> TKFSDNYDVKEELGKGAFSVVRRCVHKTTGLEFAAKIINTKKLSARDFQKLEREARICRKLQHPNIVRLHDSIQEESFHYLVFDLVT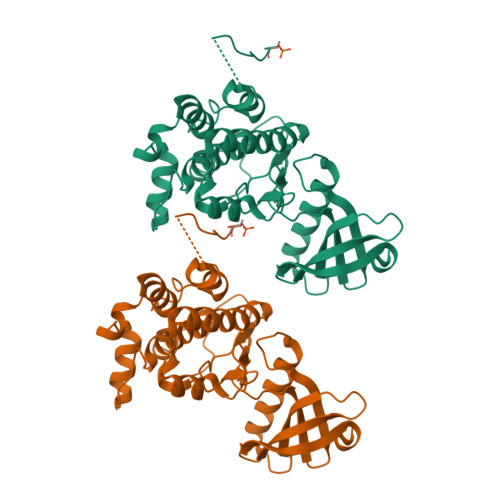GGELFEDIVAREFYSEADASHCIQQILESIAYCHSNGIVHRNLKPENLLLASKAKGAAVKLADFGLAIEVNDSEAWHGFAGTPGYLSPEVLKKDPYSKPVDIWACGVILYILLVGYPPFWDEDQHRLYAQIKAGAYDYPSPEWDTVTPEAKSLIDSMLTVNPKKRITADQALKVPWICNRERVASAIHRQDTVDC>[3x]VRIALKKRPIDRNSRVATGLSGGEEQPLLSGANPLRSEEEGDIVALKNYMNAQYFGEIGVGTPPQKFTVIFDTGSSNLWVPSAKCYFSIACYLHSRYKAGASSTYKKNGKPAAIQYGTGSIAGYFSEDSVTVGDLVVKDQEFIEATKEPGITFL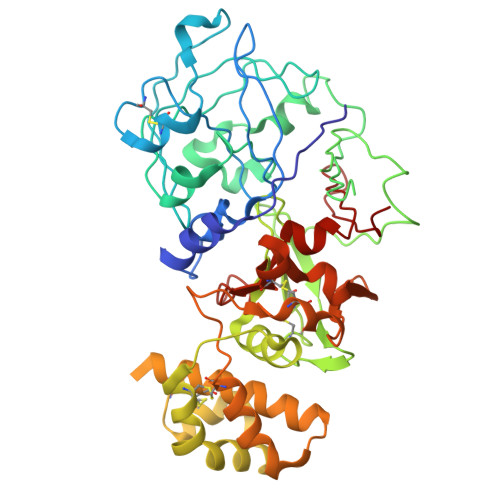VAKFDGILGLGFKEISVGKAVPVWYKMIEQGLVSDPVFSFWLNRHVDEGEGGEIIFGGMDPKHYVGEHTYVPVTQKGYWQFDMGDVLVGGKSTGFCAGGCAAIADSGTSLLAGPTAIITEINEKIGAAGVVSQECKTIVSQYGQQILDLLLAETQPKKICSQVGLCTFDGTRGVSAGIRSVVDDEPVKSNGLRADPMCSACEMAVVWMQNQLAQNKTQDLILDYVNQLCNRLPSPMGESAVDCGSLGSMPDIEFTIGGKKFALKPEEYILKVGEGAAAQCISGFTAMDIPPPRGPLWILGDVFMGPYHTVFDYGKLRIGFAKAA Microrchidia CW-type zinc finger proteins (MORCs) are a family of transcriptional regulators conserved in eukaryotes. We recently showed that human MORC2 is necessary, in conjunction with the human silencing hub (HUSH), for silencing of transgenes integrated at chromatin loci with histone H3 trimethylated at lysine 9 H3K9me3. MORC2 is a 1032-amino acid protein predicted to contain several functional domains including an N-terminal GHKL-type ATPase module with a coiled-coil insertion (CC1). Here we report the biochemical and cellular activities of MORC2 variants, alongside structures of wild-type and neuropathic variant forms of a MORC2 fragment comprising the GHKL-type ATPase module and CW domain.

We obtained crystals of human MORC2(1–603) in the presence of a molar excess of AMPPNP. The overall architecture of the crystallized MORC2 fragment bound to AMPPNP is an almost symmetric, parallel homodimer resembling the letter M. A 2778 Å2 surface from each monomer is buried at the dimer interface. One AMPPNP molecule, stabilized by an octahedrally coordinated Mg2+ ion, is bound in the active site of both protomers. In the wild-type MORC2 structure, the ATP lid (residues 82–103) is in the closed conformation in both protomers, leaving only a narrow channel between the bound AMPPNP and the solvent. Residues in the lid form a significant part of the dimer interface, with Ile82, Phe84, Arg90, Tyr100, and Asn102-forming hydrogen bonds and hydrophobic contacts with residues 12–24 of the other protomer. Notably, the β-sheet in the transducer-like domain contains an 80-amino acid antiparallel coiled-coil insertion, CC1 (residues 282–361), which forms a 6-nm projection emerging from the ATPase module. A tetrahedrally coordinated zinc atom carried over from the purification was observed bound to the CW domain. The orientation of the CW domain relative to the ATPase module differs by approximately 180˚ in the MORC2 and MORC3 structures, with the degenerate histone-binding site of the MORC2 CW domain facing toward the ATPase module rather than toward solvent. The CW domain binds an array of arginine residues in the transducer-like domain: conserved residue Trp505, providing the ‘right wall’ of the methyl-lysine-coordinating aromatic cage, forms a cation–π interaction with the sidechain of Arg266.

>[2x]GPRMAFTNYSSLNRAQLTFEYLHTNSTTHEFLFGALAELVDNARDADATRIDIYAERREDLRGGFMLCFLDDGAGMDPSDAASVIQFGKSAKRTPESTQIGQYGNGLKSGSMRIGKDFILFTKKEDTMTCLFLSRTFHEEEGIDEVIVPLPTWNARTREPVTDNVEKFAIETELIYKYSPFRTEEEVMTQFMKIPGDSGTLVIIFNLKLMDNGEPELDIISNPRDIQMAETSPEGTKPERRSFRAYAAVLYIDPRMRIFIHGHKVQTKRLSCCLYKPRMYKYTSSRFKTRAEQEVKKAEHVARIAEEKAREAESKARTLEVRLGGDLTRDSRVMLRQVQNRAITLRREADVKKRIKEAKQRALKEPKELNFVFGVNIEHRDLDGMFIYNCSRLIKMYEKVGPQLEGGMACGGVVGVVDVPYLVLEPTHNKQDFADAKEYRHLLRAMGEHLAQYWKDIAIAQRGIIKFWDEFGYLSANWNQPPSSELRYKRRRAMEIPTTIQCDLCLKWRTLPFQLSSVEKDYPDTWVCSMNPDPEQDRCEASEQKQKVPLGTFRKDMKTQEEKQKQLTEKIRQQQEKLEALQKTTPIRSQADLKKLPLEVTTRPST>[4x]GHMTRFALTGLAGYIAPRHLKAIKEVGGVLVASLDPATNVGLVDSFFPEAEFFTEPEAFEAYLEDLRDRGEGVDYLSIASPNHLHYPQIRMALRLGANALSEKPLVLWPEEIARLKELEARTGRRVYTVLQLRVHPSLLALKERLGQEKGAKDVVLTYVTGRGKWYGKSWKVDEAKSGGLATNIGIHFFDLLAWLFGRALHVEVHARTPTVNAGYL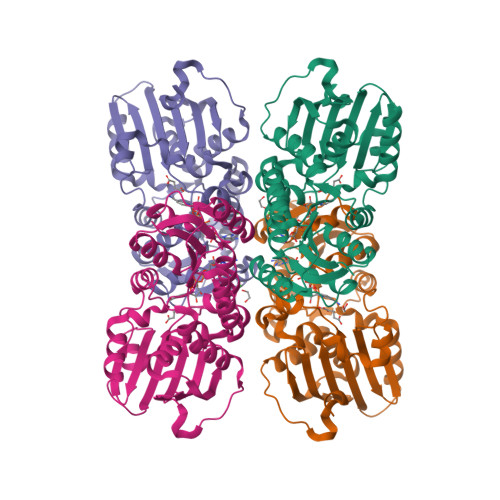ELEGARVRWFLSIDPSFVPEPLRRQGKRTYRSIAVDGEEVEFSEGFTDLHTEVYRKTLAGEGFGLDEAAEAIRVAALLRTLPLSQPSPENRHPFLG>MHHHHHHNEEFRPEMLQGKKVIVTGASKGIGREMAYHLSKMGAHVVLTARSEEGLQKVVSRCLELGAASAHYIAGTMEDMTFAEQFIVKAGKLMGGLDMLILNHITQTSLSLFHDDIHSVRRVMEVNFLSYVVMSTAALPMLKQSNGSIAVISSLAGKMTQPMIAPYSASKFALDGFFSTIRTELYITKVNVSITLCVLGLIDTETAMKEISGIINAQASPKEECALEIIKGTALRKSEVYYDKSPLTPILLGNPGRKIMEFFSLR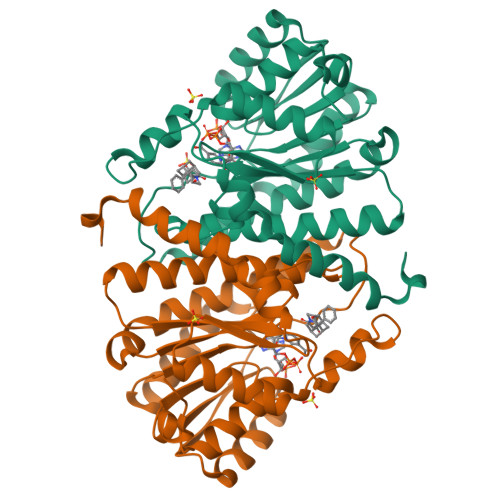YYNKDMFVSN[2x]1-(trans-4-{[7-oxo-8-(propan-2-yl)-7,8-dihydropyrido[2,3-d]pyrimidin-2-yl]amino}cyclohexyl)-3-propan-2-ylurea | C20 H30 N6 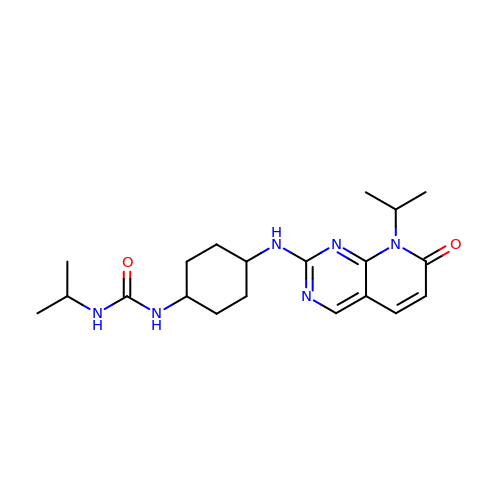O2 | FJVVBMGXZMJPOI-WKILWMFISA-N>[2x]MIGELVKDKILIKNIEDARLIYKMGYYGKPIGISKPKS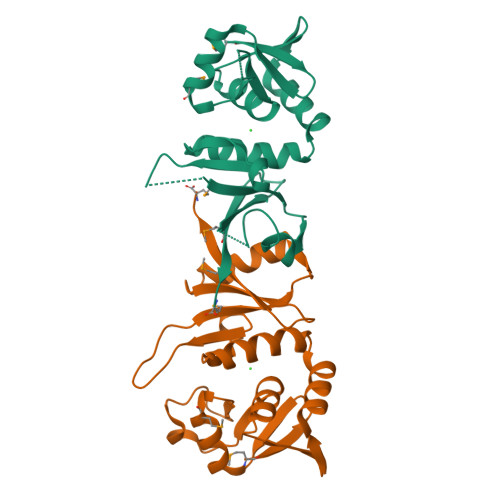AEEINSELILSLIEGVYLVKKGKLEIVSNGERLDFERLYQIGVTQIPRFRILYSVYEDLREKGYVVRSGIKYGADFAVYTIGPGIEHAPYLVIALDENSQISSNEILGFGRVSHSTRKELILGIVNLTNGKIRYIMFKWLKM>SIGLALLLLLLALLFWLYIVMSNWTGGALLVLYSFALMLIIIILIIFIFRRDLLCPLGGLGLLLLMITLLLIALWNLHGQALYLGIVLFIFGCLLVLGLWIYFLEILWRLGATIWQLLAFILAFFLAIILLIIALYLQQNWWTLLVDLLWLLLFMAILIWM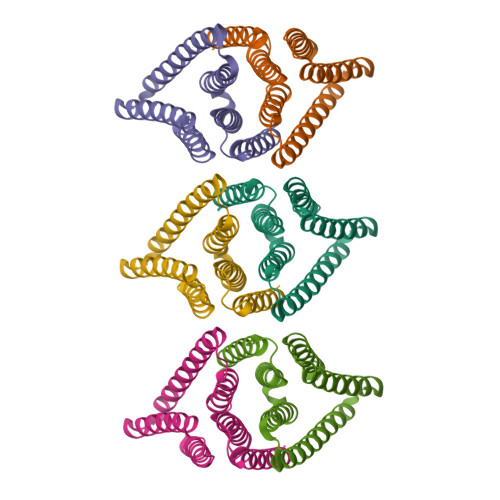Y[6x]> MDFDMIEEKKDSVIVRNVENFELKDIFDCGQCFRWHRQENGNYIGIAFEK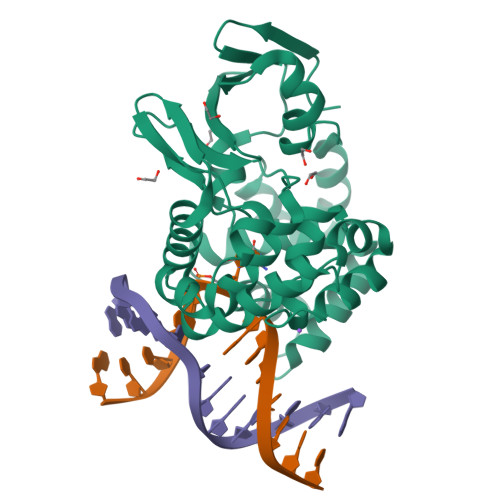VVEVQKIGEDVVIYNINEEEFKNVWSEYFDLYRDYGEIKKELSRDPLLKKSVDFGEGIRILRQDPFEILLSFIISANNRIPMIKKCINNISEKAGKKLEYKGKIYYAFPTVDKLHEFTEKDFEECTAGFRAKYLKDTVDRIYNGELNLEYIKSLNDNECHEELKKFMGVGPQVADCIMLFSMQKYSAFPVDTWVKKAMMSLYVAPDVSLKKIRDFGREKFGSLSGFAQQYLFYYARENNI>MGIPADNLQSRAKASFDTRVAAAELALNRGVVPSFANGEELLXRNPDPDNTDPSFIASFTKGLPHDDNGAIIDPDDFLAFVRAINSGDEKEIADLTLGPARDPETGLPIWRSDLANSLELEVRGWENSSAGLTFDLEGPDAQSIAMPPAPVLTSPELVAEIAELYLMALGREIEFSEFDSPKNAEXIQFAIDQLNGLEWFNTPAKLGDPPAEIRRRRGEVTVGNLFRGILPGSEVGPYLSQYIIVGSKQIGSATVGNKTLVSPNAADEFDGEIAYGSITISQRVRIATPGRDFMTDLKVFLDVQDAADFRGFESYEPGARLIRTIRDLATWVHFDALYEAYLNACLILLANGVPFDPNLPFQQEDKLDNQDVFVNFGSAHVLSLVTEVATRALKAVWYQKFNIHRRLRPEATGGLISVNKIAAQKGESIFPEVDLAVEELGDILEKAEISNRKQNIADGDPDPDPSFLLPMAFAEGSPFHPSYGSGHAVVAGACVTILKAFFDSGIEIDQVFEVDKDEDKLVKSSFKGTLTVAGELNKLADNIAIGRNM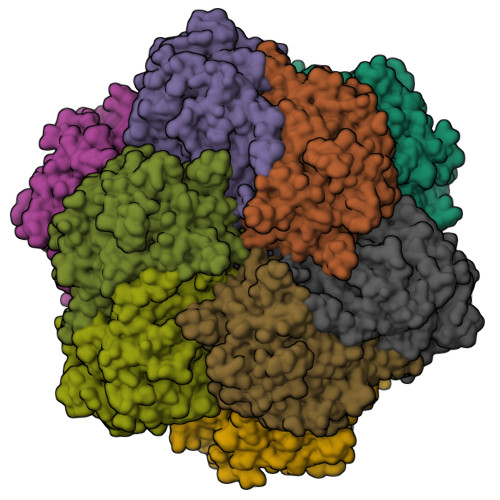AGVHYFSDQFESLLLGEQVAIGILEEQSLTYGENFFFNLPKFDGTTIQI[4x]>[2x]MALVYDAEFVGSEREFEEERETFLKGVKAYDGVLATRYLMERSSSAKNDEELLELHQNFILLTGSYACSIDPTEDRYQNVIVRGVNFDERVQRLSTGGSPARYAIVYRRGWRAIAKALDIDEEDVPAIEVRAVKRNPLQPALYRILVRYGRVDLMPVTVDEVPPEMAGEFERLIERYDVPIDEKEERILEILRENPWTPHDEIARRLGLSVSEVEGEKDPESSGIYSLWSRVVVNIEYDERTAKRHVKRRDRLLEELYEHLEELSERYLRHPLTRRWIVEHKRDIMRRYLEQRIVECALKLQDRYGIREDVALCLARAFDGSISMIATTPYRTLKDVCP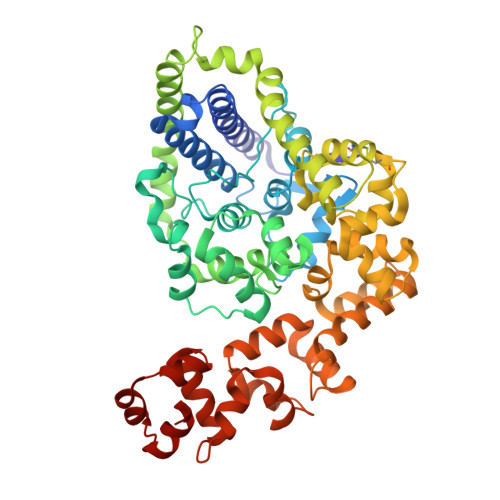DLTLEEAKSVNRTLATLIDEHGLSPDAADELIEHFESIAGILATDLEEIERMYEEGRLSEEAYRAAVEIQLAELTKKEGVGRKTAERLLRAFGNPERVKQLAREFEIEKLASVEGVGERVLRSLVPGYASLISIRGIDRERAERLLKKYGGYSKVREAGVEELREDGLTDAQIRELKGLK>[2x]MNSSLPSLRDVFANDFRIGAAVNPVTIEMQKQLLIDHVNSITAENHMKFEHLQPEEGKFTFQEADRIVDFACSHRMAVRGHTLVWHNQTPDWVFQDGQGHFVSRDVLLERMKCHISTVVRRYKGKIYCWDVINEAVADEGNELLRPSKWRQIIGDDFMEQAFLYAYEADPDALLFYNDYNECFPEKREKIFALV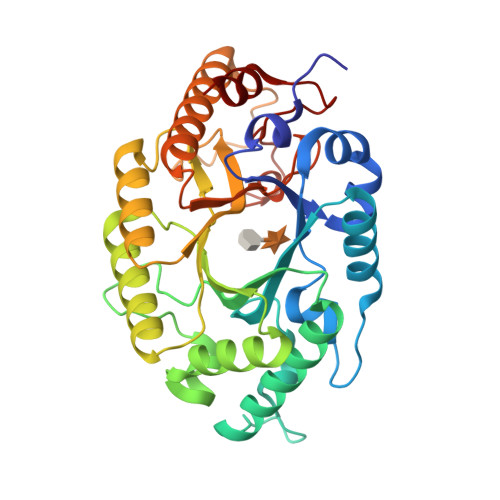KSLRDKGIPIHGIGMQAHWSLTRPSLDEIRAAIERYASLGVVLHITGLDVSMFEFHDRRTDLAAPTSEMIERQAERYGQIFALFKEYRDVIQSVTFWGIADDHTWLDNFPVHGRKNWPLLFDEQHKPKPAFWRAVSV>[4x]NSKDSIVNDDDDSTSEVDAIPDSTNPSGSFPSVEYDVFLSFRGPDTRKQFTDFLYHFLCYYK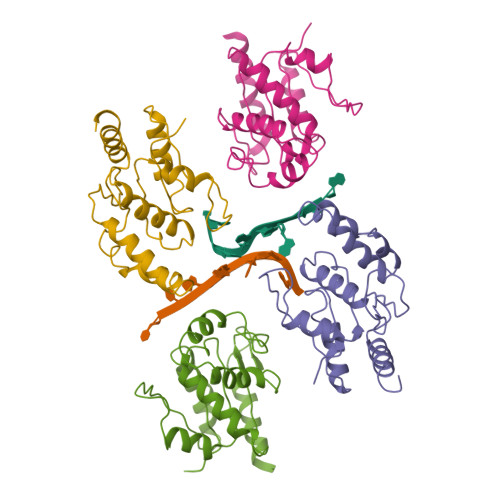IHTFRDDDELRKGKEIGPNLLRAIDQSKIYVPIISSGYADSKWCLMELAEIVRRQEEDPRRIILPIFYMVDPSDVRHQTGCYKKAFRKHANKFDGQTIQNWKDALKKVGDLKGWHIGKDDEQGAIADKVSADIWSHISKENL> GAGCAGCCTGTTTGGACATCA;> CCAUAC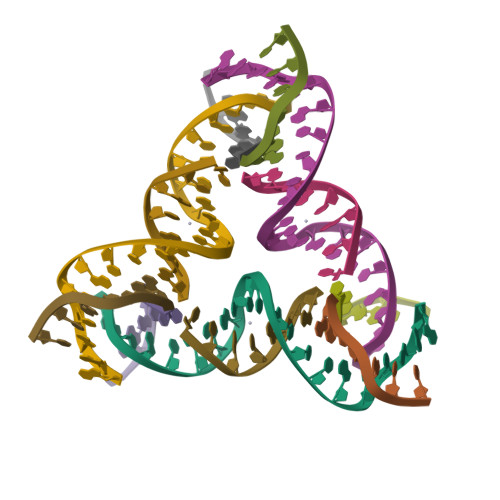A;> GGCTGCT;> CTGATGT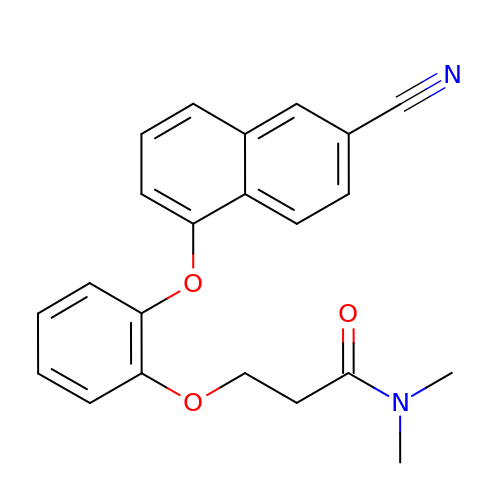3-{2-[(6-cyanonaphthalen-1-yl)oxy]phenoxy}-N,N-dimethylpropanamide | C22 H20 N2 O3 | QIORNPOXHBDSPJ-UHFFFAOYSA-N>MSDPVSYTRKDSIAVISMDDGKVNALGPAMQQALNAAIDNADRDDVGALVITGNGRVFSGGFDLKILTSGEVQPAIDMLRGGFELAYRLLSYPKPVVMACTGHAIAMGAFLLSCGDHRVAAHAYNIQANEVAIGMTIPYAALEIMKLR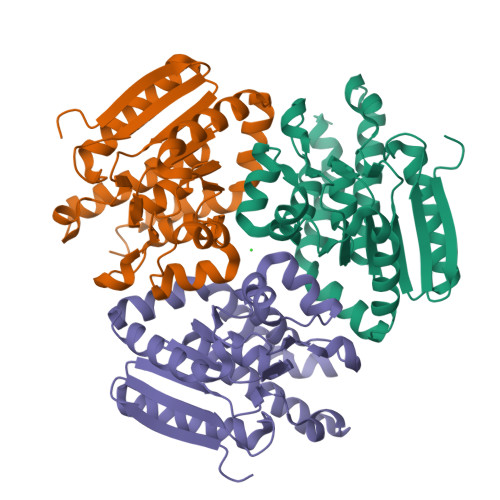LTRSAYQQATGLAKTFFGETALAAGFIDEIALPEVVVSRAEEAAREFAGLNQHAHAATKLRSRADALTAIRAGIDGIAAEFGL[3x]> GLLTPPQ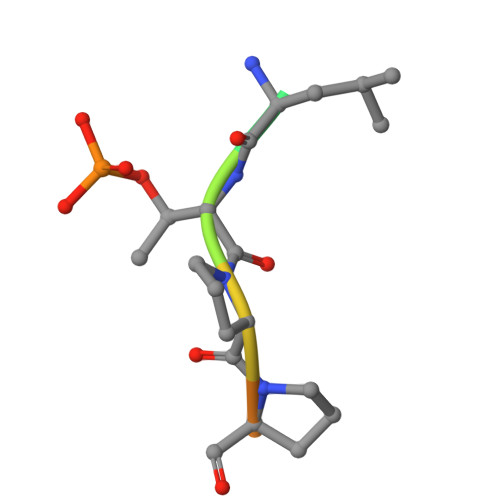SG>GEIPTIGQQMETGDQRFGDLVFRQLAPNVWQHTSYLDMPGFGAVASNGLIVRDGGRVLVVDTAWTDDQTAQILNWIKQEINLPVALAVVTHAHQDKMGGMDALHAAGIATYANALSNQLAPQEGMVAAQHSLTFAANGWVEPATAPNFGPLKVFYPGPGHTSDNITVGIDGTDIAFGGCLIKDSKAKSLGNLGDADTEHYAASARAFGAAFPKASMIVMSHSAPDSRAAITHTA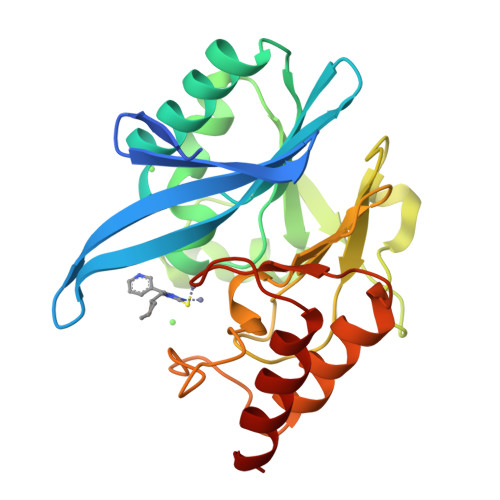RMADKLR[2x]> MEDYTLREREQEIYNRQVIKRPFDPDSYLTADLHLYLKNGKTLTIHIERNLFFSHEFTWEEICRGAYREHYLSNSGPGKCDTQEYIDGLVADNGGRSTHNSSYLEPVAFQLTLLGNFDLGSIHLRIGDYLGFRDGQRFPCKETIHGRRDTIGPFMQGMSGKWAKEDYIHTYSGRFDCKTSRHPSIFLAFMRANQDGHSSFAPENMRNALLYSGDKSPRYILMDNEHTLINNFIIPRCLPYRDQYGKDY

Cypoviruses, members of the family Reoviridae, subfamily Spinareovirus, possess a single capsid layer with turrets and are commonly embedded in crystalline occlusion bodies called polyhedra, which are formed in the cell cytoplasm and mainly composed of a single virus-encoded protein, polyhedrin. To ensure the delivery of virus particles to the target intestinal cells, allowing the transmission of packages of infectious virus between hosts by oral-faecal routes, polyhedra are disrupted only when they are exposed to the very alkaline pH environment found in insect midguts. The fold of all the polyhedrins is highly similar – a β-barrel core sitting on a base domain, surrounded by a common array of five helices (H1–H5). The strongest intermolecular interactions define a trimer composed of a cluster of three β-barrels sandwiched by helices top and bottom.

CPV15 is like CPV5, but with a smaller clamp, and has a dramatic conformational change in V4. CPV15 is similar to CPV5 however V3 and V2c are shorter, leaving space for two ATPs in different conformations to CPV1: one binds V3 and V2c and the other stacks at the 2-fold axis with the backbone of V4 forming a further layer. The full length polyhedrin structures are generally well ordered, as expected for a crystal lattice which has extensive interactions and low solvent content (19–25%), however some types show regions of flexibility: 13 residues (136–148) of CPV5 and 6 residues (68–73) of CPV14 have high (>40 compared with an overall Wilson B-factor of 21.3) B-factors, whilst 13 residues (66–78) of CPV15 could not be modelled. CPV4 has limited numbers of molecular interactions in this area, while in CPV5 a few strong trimer-trimer interactions are present. In CPV15, 13 disordered residues are situated around this region (indicated by dashed lines in Fig. 5) leaving the trimer contacts apparently weakened. The V5 regions of CPV5, 15, 17 and 19 differ, but all end in a similar place. In CPV1, 14, 15, 17, 18 and 20 solvent molecules can move between these two voids, whereas in CPV4, 5 and 19 they are blocked by tyrosine residues.>[6x]APAVAHHHHHHAVADKADNAFMMICTALVLFMTIPGIALFYGGLIRGKNVLSMLTQVTVTFALVCILWVVYGYSLAFGEGNNFFGNINWLMLKNIELTAVMGSIYQYIHVAFQGSFACITVGLIVGALAERIRFSAVLIFVVVWLTLSYIPIAHMVWGGGLLASHGALDFAGGTVVHINAAIAGLVGAYLIGKRVGFGKEAFKPHNLPMVFTGTAILYIGWFGFNAGSAGTANEIAALAFVNTVVATAAAILGWIFGEWALRGKPSLLGACSGAIAGLVGVTPACGYIGVGGALIIGVVAGL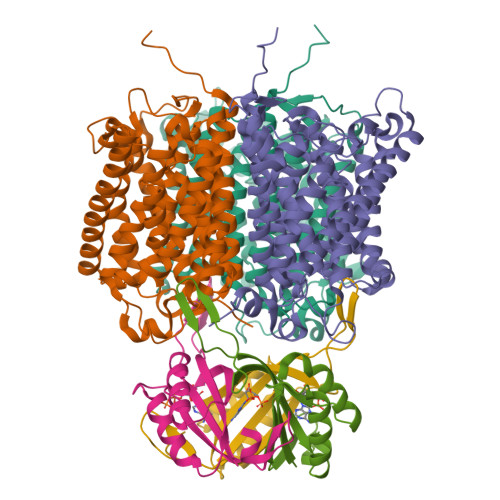AGLWGVTMLKRLLRVDDPCDVFGVHGVCGIVGCIMTGIFAASSLGGVGFAEGVTMGHQLLVQLESIAITIVWSGVVAFIGYKLADLTVGLRVPEEQEREGLDVNSHGENAYNA;>[6x]MKLVTVIIKPFKLEDVREALSSIGIQGLTVTEVKGFGRQKGHAELYRGAEYSVNFLPKVKIDVAIADDQLDEVIDIVSKAAYTGKIGDGKIFVAELQRVIRIRTGEADEAAL> EPVMTGGPVQGKALWTDYSGMSKEVQGPVSQILFTQSPRTAKGDPYQNYPHYIPEGSRIVLFDLNTKELKVLTNDFATAFDPCTYWDGKKFAFAGVHKKGGGCQIWEMNIDGSGLRQMTDLKGTCRSPIYYAAGSIEEGEGRIIWRDRYFEGDWKEHGMVEKTGMIIFSGSPEGVMDEFHNPYAYNLYRLDTQGGKIIQRITGHVLSGIEFPHLNTTIDQITYNLSSNFDPWLTPDGNILFS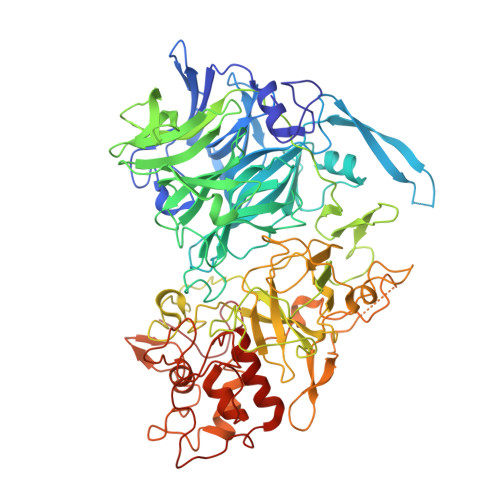SVQANGSRAGGEGRVMICVDNWDGAYPRPIYGNCDGEIGGTSGRSQAKITFGDRKIVYVESPYMNWGVGQLAAVSWDAPFNKTYEKLTGKDGGLYRSPYPLPDDRMLVSYAERGDFGIYWFNFSKCAAGDKVYDDPNWNDHQPAPVYVKYKPRWINTFTAGKNFGVTVVTYQPFDQVKVEGYPHSWGTWICFDTTLSDQPVGPYPHQKAKNVSHGDIKAVRIIQGYQCVEPDSTRFRVGAGAHLLGGERSSSNSGTAFQQRGIIGYQYVESDGSTVTSQLSDVPYYMQILDDKGMSVQTALTWAYLRPYHGRICSGCHYGSYRGRAFKNIHAKALYNWWYDDRSHYDSPFAFRYLKFDNDGNYKGVKHGEDVVVPSDIYYGGPSGTTSQPVEGLTLDKQRTVDFRRDIQPILDAKCAMCHDSNNPPNLGGGLELVSVDGIAAYSRAYNSLLEPQRGKDPNIGGKYVNPSAAINSLLVWRLYEAELSANAPREKIFPIEGRLLHNKFLTQDERYAIVEWIDLGAQWDNIPGPDFYPGYLVK> EGLTIDLKNFRKPGEKTFTQRSRLFVGNLPPDITEEEMRKLFEKYGKAGEVFIHKDKGFGFI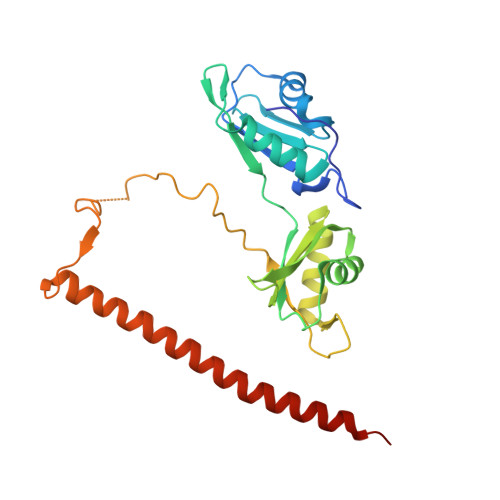RLETRTLAEIAKVELDNMPLRGKQLRVRFACHSASLTVRNLPQYVSNELLEEAFSVFGQVERAVVIVDDRGRPSGKGIVEFSGKPAARKALDRCSEGSFLLTTFPRPVTVEPMDQLDDEEGLPEKLVIKNQQFHKEREQPPRFAQPGSFEYEYAMRWKALIEMEKQQQDQVDRNIKEAREKLEMEMEAARHEHQVMLM>[2x]XTTLSDKDKSTVKA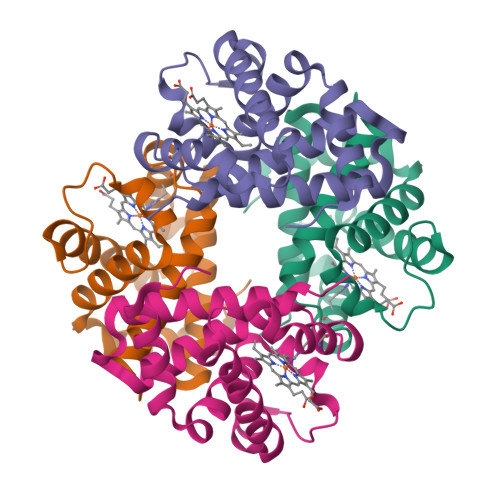LWGKISKSADAIGADALGRMLAVYPQTKTYFSHWPDMSPGSGPVKAHGKKVMGGVALAVSKIDDLTTGLGDLSELHAFKMRVDPSNFKILSHCILVVVAKMFPKEFTPDAHVSLDKFLASVALALAERYR;>VEWTQQERSIIAGIFANLNYEDIGPKALARCLIVYPWTQRYFGAYGDLSTPDAIKGNAKIAAHGVKVLHGLDRAVKNMDNINEAYSELSVLHSDKLHVDPDNFRILGDCLTVVIAANLGDAFTVETQCAFQKFLAVVVFALGRKYH[2x]(1~{S},5~{S},6~{R})-10-[3,5-bis(chloranyl)phenyl]sulfinyl-5-ethenyl-3-(pyridin-2-ylmethyl)-3,10-diazabicyclo[4.3.1]decan-2-one 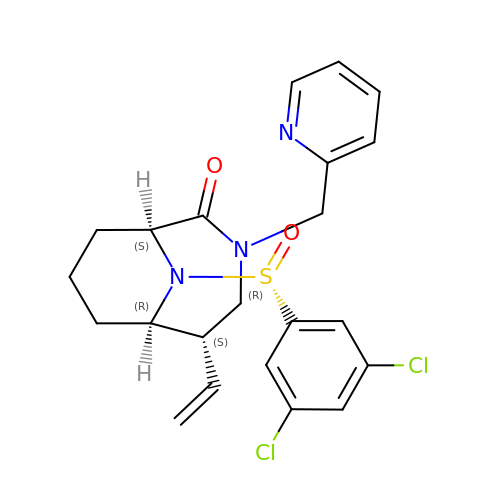| C22 H23 Cl2 N3 O2 S | YFTZNIHUDDONNU-MIQCLTDXSA-N Galectins are multi-purpose effectors acting via interactions with distinct counterreceptors based on protein-glycan/protein recognition. We report here the first crystallographic information on the N-terminal extension of the carbohydrate recognition domain of rat galectin-5, which is precisely described as an N-tailed proto-type-like galectin. The overall fold in ligand-free and -loaded rGal-5 is composed of two antiparallel β-sheets (F1 to F5 and S1 to S6 strands) that form the characteristic β-sandwich structure. The presented data shows that the N-terminal extension can adopt an ordered structure and shapes the hypothesis that a ligand-induced shift in the equilibrium between flexible and ordered conformers potentially acts as a molecular switch, enabling new contacts in this region.

The rGal-5–lactose complex crystals belong to space group P22121, with only two molecules present in the asymmetric unit, and diffract to a 1.9 Å resolution. The two CRDs present in the asymmetric unit, which have bound lactose (Lac), exhibit very similar features to ligand-free rGal-5, with an RMSD value of only 0.3 Å for all Cα atoms. One of the two monomers in the asymmetric unit exhibits strong electron density for the first 10 residues so that their structure could be modelled. Intriguingly, these residues run parallel to the edge of the β-sandwich instead of forming the F0 strand and the protuberant loop observed in the ligand-free state. Intramolecular (hydrogen bonds between Ser2 and Ser3 with Ser39) and intermolecular contacts with symmetry-related molecules (hydrogen bond between Thr6 and Asp40) stabilize this special spatial arrangement. The carbohydrate-binding site in the concave face of the β-sheet is constituted by β-strands S4 to S6. The amino acids of the signature sequence, i.e., His57, Asn59, Arg61, Asn70, Glu80 and Arg82, directly interact with lactose through hydrogen bonding interactions. Additionally, Arg43, Gln45 and Glu64 form water-mediated hydrogen bonds with the ligand. As commonly found in galectin–lactose complexes, the indole ring of Trp77 stacks to the β-face of the pyranose ring of galactose. rGal-5 interact with Lac with a dissociation constant of 136 ± 16 μM, which is lowered in the case of LacNAc to 30.5 ± 1.9 μM and 5.5 ± 0.6 μM for the blood-group B tetrasaccharide.

>[2x]MSSFSTQTPYPNLAVPFFTSIPNGLYPSKSIVISGVVLSDAKRFQINLRCGGDIAFHLNPRFDENAVVRNTQINNSWGPEERSLPGSMPFSRGQRFSVWILCEGHCFKVAVDGQHICEYSHRLMNLPDINTLEVAGDIQLTHVET> SLGVQPPNFSWVLPGRLAGLALPRLPAHYQFLLDLGVRHLVSLTERGPPHSDSCPGLTLHRLRIPDFCPPAPDQIDRFVQIVDEANARGEAVGVHCALGFGRTGTMLACYLVKERGLAAGDAIAEIRRLRPGSIETYEQEKAV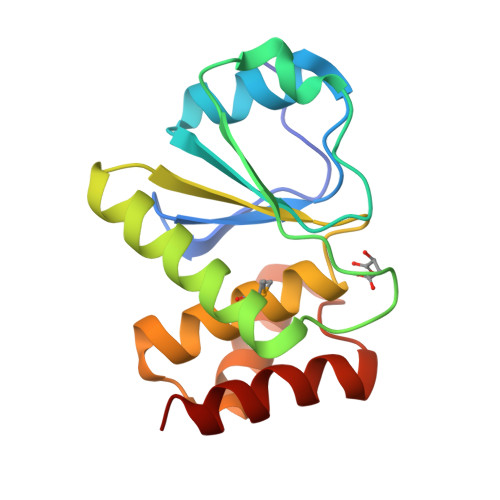FQFYQRTK The particles harbour 10-separate genome segments and comprise two principle protein layers, the innermost composed of 120 copies of protein λ1 clamped together by 150 copies of σ2 (viral polymerases, λ3, are attached inside adjacent to the icosahedral fivefold axes). The outer layer consists of 600 copies each of μ1 and σ3. The array of μ1 and σ3 is interrupted at the fivefold axes by pentameric λ2 turrets which enzymatically cap the mRNA transcripts produced by the polymerase on egress from the particle. Here we demonstrate that vitrification of infected cells followed by cryo-focussed ion beam (cryo-FIB) milling and cryo-electron tomography (cryo-ET) allows high resolution reconstruction of assembly intermediates of a mammalian reovirus, allowing atomic models to be constructed which throw light on some of these fundamental questions.

In addition virion-like particles of two types, ‘empty’ and ‘full’, were observed. For stars, analysis focused on the fivefold regions using emClarity16 yielded a reconstruction at 6.6 Å. For the empty virion-like particles, reconstructions focused on the fivefold regions and pseudo sixfold regions yielded reconstructions at 6.5 and 5.6 Å respectively. Thus purified virus particles provide a good model for the in-cell empty virion-like particle indicating that the internal RNA does not alter the fundamental organisation of the structure, thus at the fivefold axis on the exterior of the particle, there is evidence for the σ1 spike being attached. Although there is essentially no RNA in these empty particles there is evidence that the λ3 polymerase is attached at the expected position to the interior of λ1 close to the fivefold axis. However there is no evidence for the lattice-work organisation of the N-terminal 181 residues of λ1 B subunits on the inside of the particle which has been assumed to play a role in organising their assembly around the threefold axes, indeed there is no evidence for ordered structure for the first 259 residues of the B subunit (in the A subunit there is density for residue 241 onwards). It is possible that these termini play a role in interactions with, and possibly organising, the genome in the mature virus. The observation of only the SLP and completely assembled virion-like particles suggests that the conversion from the SLP to a virus-type structure occurs through the relatively rapid addition of all the remaining structural components of the virus.

> NKKTAQLLHADTPRLVTWDAGLCTSFKIVPIVPAQVPQDVLAYTFFTSSYAIQSPFPEAAVSRIVVHTRWASNVDFDRDSSVIMAPPTENNIHLFKQLLNTETLSVRGANPLMFRANVLHMLLEFVLDNLYLNRHTGFSQDHTPFTEGANLRSLPGPDAEKWYSIMYPTRMGTPNVSKICNFVASCVRNRVGRFDRAQMMNGAMSEWVDVFETSDALTVSIRGRWMARLARMNINPTEIEWALTECAQGYVTVTSPYAPSVNRLMPYRISNAERQISQIIRIMNIGNNATVIQPVLQDISVLLQRISPLQIDPTIISNTMSTVSESTTQTLSPASSILGKLRPSNSDFSSFRVALAGWLYNGVVTTVIDDSSYPKDGGSVTSLENLWDFFILALALPLTTDPCAPVKAFMTLANMMVGFETIPMDNQIYTQSRRASAFSTPHTWPRCFMNIQLISPIDAPILRQWAEIIHRYWPNPSQIRYGAPNVFGSANLFTPPEVLLLPIDHQPANVTTPTLDFTNELTNWRARVCELMKNLVDNQRYQPGWTQSLVSSMRGTLDKLKLIKSMTPMYLQQLAPVELAVIAPMLPFPPFQVPYVRLDRDRVPTMVGVTRQSRDTITQPALSLSTTNTTVGVPLALDARAITVALLSGKYPPDLVTNVWYADAIYPMYADTEVFSNLQRDMITCEAVQTLVTLVAQISETQYPVDRYLDWIPSLRASAATAATFAEWVNTSMKTAFDLSDMLLEPLLSGDPRMTQLAIQYQQYNGRTFNVIPEMPGSVIADCVQLTAEVFNHEYNLFGIARGDIIIGRVQSTHLWSPLAPPPDLVFDRDTPGVHIFGRDCRISFGMNGAAPMIRDETGMMVPFEGNWIFPLALWQMNTRYFNQQFDAWIKTGELRIRIEMGAYPYMLHYYDPRQYANAWNLTSAWLEEITPTSIPSVPFMVPISSDHDISSAPAVQYIISTEYNDRSLFCTNSSSPQTIAGPDKHIPVERYNILTNPDAPPTQIQLPEVVDLYNVVTRYAYETPPITAVVMGVP;> AGLCTSFKIVPIVPAQVPQDVLAYTFFTSSYAIQSPFPEAAVSRIVVHTRWASNVDFDRDSSVIMAPPTENNIHLFKQLLNTETLSVRGANPLMFRANVLHMLLEFVLDNLYLNRHTGFSQDHTPFTEGANLRSLPGPDAEKWYSIMYPTRMGTPNVSKICNFVASCVRNRVGRFDRAQMMNGAMSEWVDVFETSDALTVSIRGRWMARLARMNINPTEIEWALTECAQGYVTVTSPYAPSVNRLMPYRISNAERQISQIIRIMNIGNNATVIQPVLQDISVLLQRISPLQIDPTIISNTMSTLSPASSILGKLRPSNSDFSSFRVALAGWLYNGVVTTVIDDSSYPKDGGSVTSLENLWDFFILALALPLTTDPCAPVKAFMTLANMMVGFETIPMDNQIYTQSRRASAFSTPHTWPRCFMNIQLISPIDAPILRQWAEIIHRYWPNPSQIRYGAPNVFGSANLFTPPEVLLLPIDHQPANVTTPTLDFTNELTNWRARVCELMKNLVDNQRYQPGWTQSLVSSMRGTLDKLKLIKSMTPMYLQQLAPVELAVIAPMLPFPPFQVPYVRLDRDRVPTMVGVTRQSRDTITQPALSLSTTNTTVGVPLALDARAITVALLSGKYPPDLVTNVWYADAIYPMYADTEVFSNLQRDMITCEAVQTLVTLVAQISETQYPVDRYLDWIPSLRASAATAATFAEWVNTSMKTAFDLSDMLLEPLLSGDPRMTQLAIQYQQYNGRTFNVIPEMPGSVIADCVQLTAEVFNHEYNLFGIARGDIIIGRVQSTHLWSPLAPPPDLVFDRDTPGVHIFGRDCRISFGMNGAAPMIRDETGMMVPFEGNWIFPLALWQMNTRYFNQQFDAWIKTGELRIRIEMGAYPYMLHYYDPRQYANAWNLTSAWLEEITPTSIPSVPFMVPISSDHDISSAPAVQYIISTEYNDRSLFCTNSSSPQTIAGPDKHIPVERYNILTNPDAPPTQIQLPEVVDLYNVVTRYAYETPPITAVVMGVP;>[2x]ARAAFLFKTVGFGGLQNVPINDELSSHLLRAGNSPWQLTQFLDWISLGRGLATSALVPTAGSRYYQMSCLLSGTLQIPFRPNHRWGDIRFLRLVWSAPTLDGLVVAPPQVLAQPALQAQADRVYDCDDYPFLARDPRFKHRVYQQLSAVTLLNLTGFGPISYVRVDEDMWSGDVNQLLMNYFGHTFAEIAYTLCQASANRPWEHDGTYARMTQIILSLFWLSYVGVIHQQNTYRTFYFQCNRRGDAAEVWILSCSLNHSAQIRPGNRSLFVMPTSPDWNMDVNLILSSTLTGCLCSGSQLPLIDNNSVPAVSRNIHGWTGRAGNQLHGFQVRRMVTEFCDRLRRDGVMTQAQQNQIEALADQTQQFKRDKLEAWAREDDQYNQANPNSTMFRTKPFTNAQWGRGNTGATSAAIAALI;>[3x]TINVTGDGNVFKPSAETSSTAVPSLSLSPGMLNPGGVPWIAIGDETSVTSPGALRRMTSKDIDEPLVVVTEHAIANFTKAEMALEFNREFLDKLRVLSVSPKYSDLLTYVDCYVGVSARQALNNFQKQVPVITPTRQTMYVDSIQAALKALEKWEIDLRVAQTLLPTNVPIGEVSCPMQSVVKLLDDQLPDDSLIRRYPKEAAVALAKRNGGIQWMDVSEGTVMNEAVNAVAASALAPSASAPPLEEKSKLTEQAMDLVTAAEPEIIASLVPVPAPVFAIPPKPADYNVRTLKIDEATWLRMIPKTMGTLFQIQVTDNTGTNWHFNLRGGTRVVNLDQIAPMRFVLDLGGKSYKETSWDPNGKKVGFIVFQSKIPFELWTAASQIGQATVVNYVQLYAEDSSFTAQSIIATTSLAYNYEPEQLNKTDPEMNYYLLATFIDSAAITPTNMTQPDVWDALLTMSPLSAGEVTVKGAVVSEVVPAELIGSYTPESLNASLPNDAARCMIDRASKIAEAIKIDDDAGPDEYSPNSVPIQGQLAISQLETGYGVRIFNPKGILSKIASRAMQAFIGDPSTIITQAAPVLSDKNNWIALAQGVKTSLRTKSLSAGVKTAVSKLSSSESIQNWTQGFLDKVSTHFPAP;> ANVWGVRLADSLSSPTIETRTRQYTLHDLCSDLDANPGREPWKPLRNQRTNNIVAVQLFRPLQGLVLDTQLYGFPGAFDDWERFMREKLRVLKYEVLRIYPISNYSNEHVNVFVANALVGAFLSNQAFYDLLPLLIINDTMIGDLLGTGASLSQFFQSHGDVLEVAAGRKYLQMENYSNDDDDPPLFAKDLSDYAKAFYSDTYEVLDRFFWTHDSSAGVLVHYDKPTNGHHYLLGTLTQMVSAPPYIINATDAMLLESCLEQFSANVRARPAQPVTRLDQCYHLRWGAQYVGEDSLTYRLGVLSLLATNGYQLARPIPRQLTNRWLSSFVSQIMSDGVNETPLWPQERYVQIAYDSPSVVDGATQYGYVRKNQLRLGMRISALQSLSDTPSPVQWLPQYTIDQAAMDEGDLMVSRLTQLPLRPDYGNIWVGDALSYYVDYNRSHRVVLSSELPQLPDTYFDGDEQYGRSLFSLARKIGDRSLVKDTAVLKHAYQAIDPNTGKEYLRSRQSVAYFGASAGHSGADQPLVIEPWIQGKISGVPPPSSVRQFGYDVARGAIVDLARPFPSGDYQFVYSDVDQVVDGHDDLSISSGLVESLLSSCMHATAPGGSFVVKINFPTRPVWHYIEQKILPNITSYMLIKPFVTNNVELFFVAFGVHQHSSLTWTSGVYFFLVDHFYRYETLSTISRQLPSFGYVDDGSSVTGIETISIENPGFSNMTQAARIGISGLCANVGNARKSIAIYESHGARVLTITSRRSPASARRKSRLRYLPLIDPRSLEVQARTILPADPVLFENVSGASPHVCLTMMYNFEVSSAVYDGDVVLDLGTGPEAKILELIPATSPVTCVDIRPTAQPSGCWNVRTTFLELDYLSDGWITGVRGDIVTCMLSLGAAAAGKSMTFDAAFQQLIKVLSKSTANVVLVQVNCPTDVVRSIKGYLEIDSTNKRYRFPKFGRDEPYSDMDALEKICRTAWPNCSITWVPLSYDLRWTRLALLESTTLSSASIRIAELMYKYMPIMRIDIHGLPMEKRGNFIVGQNCSLVIPGFNAQDVFNCYFNSALAFSTEDVNAAMIPQVSAQFDATKGEWTLDMVFSDAGIYTMQALVGSNANPVSLGSFVVDSPDVDITDAWPAQLDFTIAGTDVDITVNPYYRLMTFVRIDGQWQIANPDKFQFFSTLVMNVKLDIADKYLLYYIRDVQSRDVGFYIQHPLQLLNTITLPTNEDLFLSAPDMREWAVKESGNTICILNSQGFVLPQDWDVLTDTISWSPSIPTYIVPPGDYTLTPL;>MEVCLPNGHQIVDLINNAFEGRVSIYSAQEGWDKTISAQPDMMVCGGAVVCMHCLGVVGSLQRKLKHLPHHRCNQQIRHQDYVDVQFADRVTAHWKRGMLSFVCQMHAMMNDVSPEDLDRVRTEGGSLVELNWLQVDPNSMFRSIHSSWTDPLQVVDDLDTKLDQYWTALNLMIDSSDLVPNFMMRDPSHAFNGVRLEGDARQTQFSRTFDSRSSLEWGVMVYDYSELEHDPSKGRAYRKELVTPARDFGHFGLSHYSRATTPILGKMPAVFSGMLTGNCKMYPFIKGTAKLKTVRKLVDSVNHAWGVEKIRYALGPGGMTGWYNRTMQQAPIVLTPAALTMFSDTTKFGDLDYPVMIGDPMILG[3x]>[2x]GASSQRSVARMDGDVIIGALFSVHHQPPAEKVPERKCGEIREQYGIQRVEAMFHTLDKINADPVLLPNITLGSEIRDSCWHSSVALEQSIEFIRDSLISIRDEKDGINRCLPDGQSLPPGRTKKPIAGVIGPGSSSVAIQVQNLLQLFDIPQIAYSATSIDLSDKTLYKYFLRVVPSDTLQARAMLDIVKRYNWTYVSAVHTEGNYGESGMDAFKELAAQEGLCIAHSDKIYSNAGEKSFDRLLRKLRERLPKARVVVCFCEGMTVRGLLSAMRRLGVVGEFSLIGSDGWADRDEVIEGYEVEANGGITIKLQSPEVRSFDDYFLKLRLDTNTRNPWFPEFWQHRFQCRLPGHLLENPNFKRICTGNESLEENYVQDSKMGFVINAIYAMAHGLQNMHHALCPGHVGLCDAMKPIDGSKLLDFLIKSSFIGVSGEEVW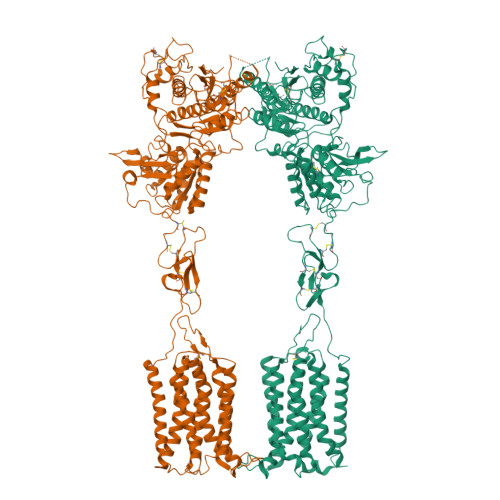FDEKGDAPGRYDIMNLQYTEANRYDYVHVGTWHEGVLNIDDYKIQMNKSGVVRSVCSEPCLKGQIKVIRKGEVSCCWICTACKENEYVQDEFTCKACDLGWWPNADLTGCEPIPVRYLEWSNIESIIAIAFSCLGILVTLFVTLIFVLYRDTPVVKSSSRELCYIILAGIFLGYVCPFTLIAKPTTTSCYLQRLLVGLSSAMCYSALVTKTNRIARILAGSKKKICTRKPRFMSAWAQVIIASILISVQLTLVVTLIIMEPPMPILSYPSIKEVYLICNTSNLGVVAPLGYNGLLIMSCTYYAFKTRNVPANFNEAKYIAFTMYTTCIIWLAFVPIYFGSNYKIITTCFAVSLSVTVALGCMFTPKMYIIIAKPERNVRSAFTTSDVVRMHVGDG[(2~{R},3~{R},4~{R},5~{R})-5-(6-aminopurin-9-yl)-3,4-diphosphonooxy-oxolan-2-yl]methyl dihydrogen phosphate | C10 H16 N5 O13 P3 | 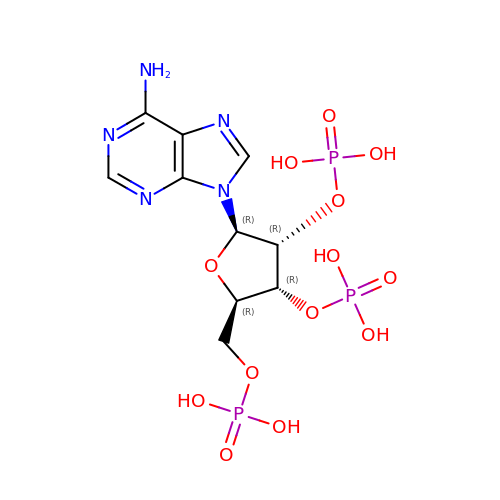JRIZSBGDMDSKRF-KQYNXXCUSA-N>[2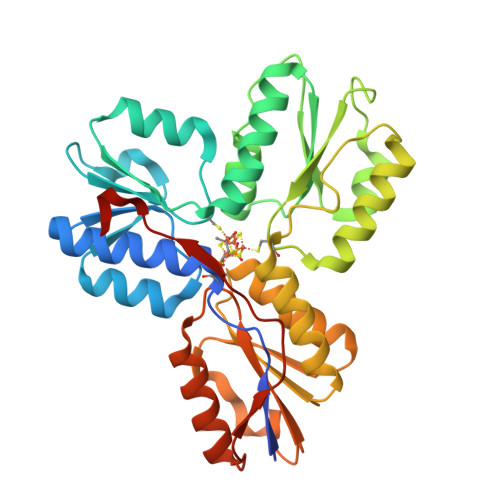x]MRGSHHHHHHGSMQILLANPRGFCAGVDRAISIVENALAIYGAPIYVRHEVVHNRYVVDSLRERGAIFIEQISEVPDGAILIFSAHGVSQAVRNEAKSRDLTVFDATCPLVTKVHMEVARASRRGEESILIGHAGHPEVEGTMGQYSNPEGGMYLVESPDDVWKLTVKNEEKLSFMTQTTLSVDDTSDVIDALRKRFPKIVGPRKDDICYATTNRQEAVRALAEQAEVVLVVGSKNSSNSNRLAELAQRMGKRAFLIDDAKDIQEEWVKEVKCVGVTAGASAPDILVQNVVARLQQLGGGEAIPLEGREENIVFEVPKELRVDIREVD> MHHHHHHVIFVAYHQKHGGYGRGGYGRQDRPQVDASRLFGESPDVVGIKKMLEGKGKQWEAIQPYFDNVVREAKNFLEWSPNKRLANAVTVAAYLTSQGLKTNQVRKILDMARTTELKV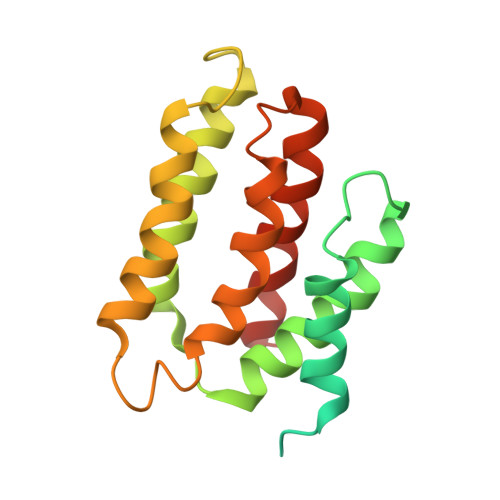KRGEGDIKDDLVKMRYLLAYTVGKATGQSKYSLDAFHRILDPMLEVLMGSPKKENFEKFYDFLQAVVAYHKFFGGGD>MSKTESYCLEDALNDLFIPETTIETILKRLTIKKNIILQGPPGVGKTFVARRLAYLLTGEKAPQRVNMVQFHQSYSYEDFIQGYRPNGVGFRRKDGIFYNFCQQAKEQPEKKYIFIIDEINRANLSKVFGEVMMLMEHDKRGENWSVPLTYSENDEERFYVPENVYIIGLMNTADRSLAVVDYALRRRFSFIDIEPGFDTPQFRNFLLNKKAEPSFVESLCQKMNELNQEISKEATILGKGFRIGHSYFCCGLEDGTSPDTQWLNEIVMTDIAPLLEEYFFDDPYKQQKWTNKLLGDSSGSHHHHHH[12x];>MEQPVIPVRNIYYMLTYAWGYLQEIKQANLEAIPGNNLLDILGYVLNKGVLQLSRRGLELDYNPNTEIIPGIKGRIEFAKTIRGFHLNHGKTVSTFDMLNEDTLANRIIKSTLAILIKHEKLNSTIRDEARSLYRKLPGISTLHLTPQHFSYLNGGKNTRYYKFVISVCKFIVNNSIPGQNKGHYRFYDFERNEKEMSLLYQKFLYEFCRRELTSANTTRSYLKWDASSISDQSLNLLPRMETDITIRSSEKILIVDAKYYKSIFSRRMGTEKFHSQNLYQLMNYLWSLKPENGENIGGLLIYPHVDTAVKHRYKINGFDIGLCTVNLGQEWPCIHQELLD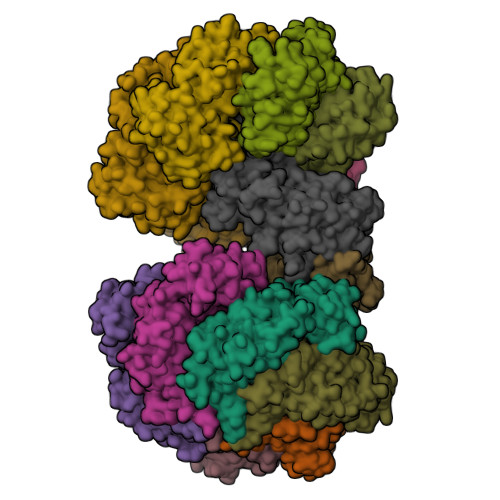IFDEYLK[2x]> MKVSTKDKIIESAVMLFNQKGFSGTSVREIAKSADVNVAHISYYFKG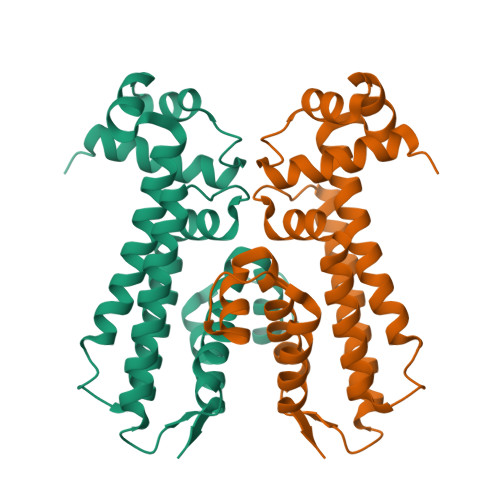KGGLMEHLVSEFYEGYSKTLETAASNISTQSTQEQLLQLVFDILSYQHNHRQLTRFVYREVTIDSTLIREIMSTYLMKEKYIFQLIIEEGEKQREYLTLPLPHFILQLKSLLMMPYLQPQYISEVLYMQPHEPYFYKMYFEEIKIWIRSVFRTGDVALTN>MIPNGYLMFEDENFIESSVAKLNALRKSGQFCDVRLQVCGHEMLAHRAVLACCSP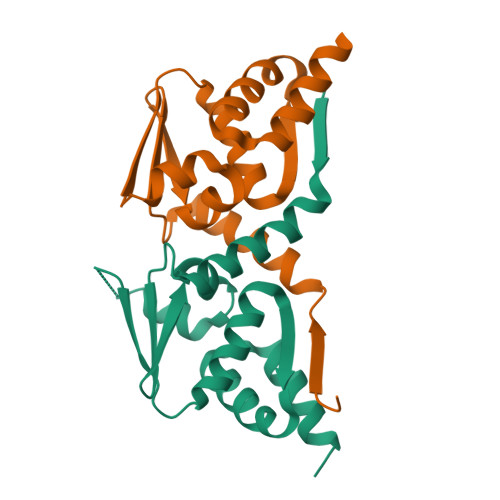YLFEIFNSDSDPHGISHVKFDDLNPEAVEVLLNYAYTAQLKADKELVKDVYSAAKKLKMDRVKQVCGDYLLSRMDVTSCISYLEHHHHHH[2x]> ATCDDGRTTANAACCILFPILDDIQENLFDGAQCGEEVHESLRLTFHDAIGFSPTLGGGGADGSIIAFDTIETNFPANAGIDEIVSAQKPFVAKHNISAGDFIQFAGAVGVSNCPGGVRIPFFLGRPDAVAASPDHLVPEPFDSVDSILARMGDAGFSPVEVVWLLASHSIAAADKVDPSIPGTPFDSTPQVFDSQFFIETQLKGRLFPGTADNKGEAQSPLQGEIRLQSDHLLARDPQTACEWQSMVNNQPKIQNRFAATMSKMALLGQDKTKLIDCSDVIPTPPALVGAAHLPAGFSLSDVEQACAATPFPALTAD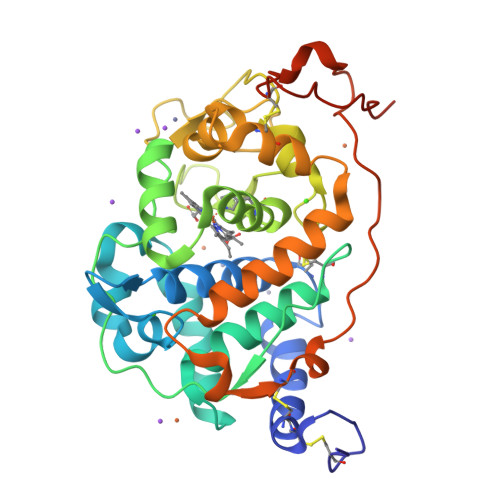PGPVTSVPPVPGS>[2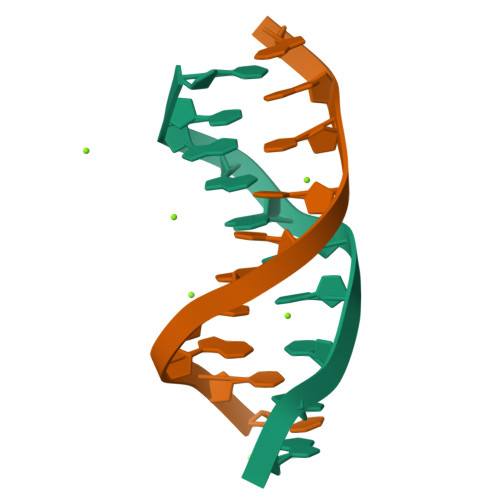x]CCAIICCTGG>[2x]MGLELFLDLVSQPSRAVYIFAKKNGIPLELRTVDLVKGQHKSKEFL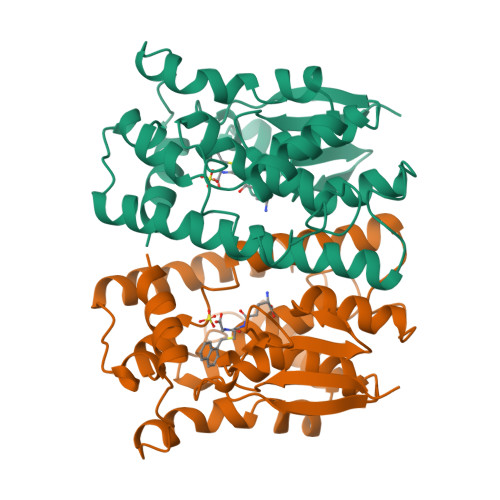QINSLGKLPTLKDGDFILTESSAILIYLSCKYQTPDHWYPSDLQARARVHEYLGWHADCIRGTFGIPLWVQVLGPLIGVQVPEEKVERNRTAMDQALQWLEDKFLGDRPFLAGQQVTLADLMALEELMQPVALGYELFEGRPRLAAWRGRVEAFLGAELCQEAHSIILSILEQAAKKTLPTPSPEAYQAMLLRIARIP> MGSSHHHHHHSSGLVPRGSHMTTTISADQVNQIIYNLHHDPFEILGCHLLEEGKNTKKWVVRAYLPKAEAAWVIRPTERKEDPMNSVHHPNFFECIIETPELNHYQLKVKEGEHEKVIYDPYAFSSPYLTDEDIYLFSEGNHHRIYEKLGAHVGEINGVKGVYFAVWAPNARNVSVIGDFNNWDGREHQMRKRNYTIWELFVPEIGSGTVYKYEIKNSEGHIYEKSDPYGFYREVRPNTASIVVDIDNIYQWHDEEWLEKRRNSDPLKQPVSVYEVHLGSWLHGSSAEKMPLLNGEADPVIVSEWNPGARFLSYYELAEKLIPYVKDMGYTHIELLPIAEHPFDGSWGYQVTGFYSPTSRFGRPEDFMYFVDKCHENGIGVILDWVPGHFPKDSHGLAYFDGTHLYEHADPRIGEHKEWGTLVFNYGRHEVRNFLVANVLFWFDKYHVDGIRVDAVASMLYRNYLRKEGEWIANEYGGDEHIEAVSFIREVNTLLFEYFPGILSIAEESTEWEKVSRPVYAGGLGFNLKWDMGWMHDMLDYFNIDPYFRQYHQNNVTFS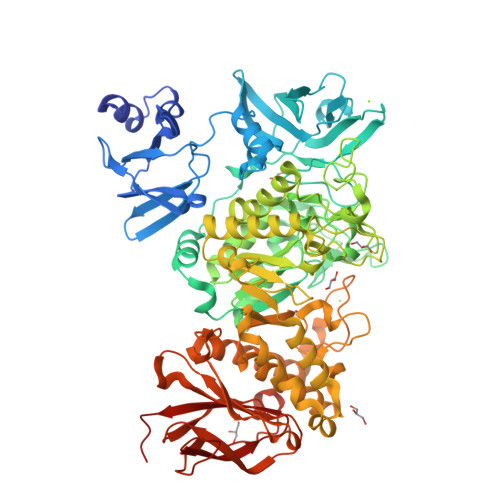MLYYYNENFMLALSHDEIVHGKSNMLGKMPGDEWQKYANVRALFTYMYTHPGKKTMFMSMEFGQWSEWNVWGDLEWHLLQYEPHQQLKQFFTDLNALYQQEPALYTHDFEYHGFEWIDCNDNTHSVVSFLRRSDDPNDSLVVVCNFTPQPHSHYRIGVPEAGYYVELFNSDAKQYGGSNMGNLGGKWADEWSFHNKPYSLDLCLPPLAVLILKLDPTKVPEGTTIKEIAADEEE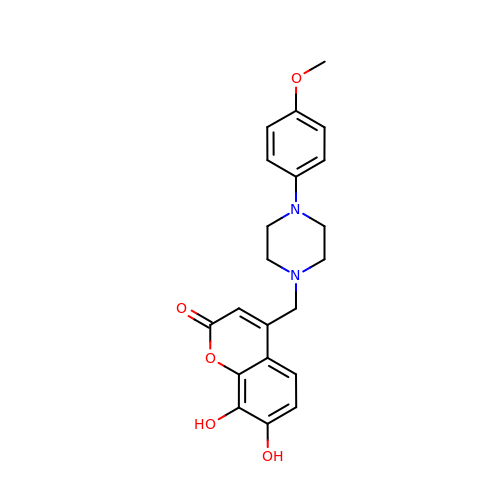4-[[4-(4-methoxyphenyl)piperazin-1-yl]methyl]-7,8-bis(oxidanyl)chromen-2-one | C21 H22 N2 O5 | NSCKGTDRMZINFP-UHFFFAOYSA-N>[2x]MGSQSTSNHLWLLSDILGQGATANVFRGRHKKTGDLFAIKVFNNISFLRPVDVQMREFEVLKKLNHKNIVKLFAIEEETTTRHKVLIMEFCPCGSLYTVLEEPSNAYGLPESEFLIVLRDVVGGM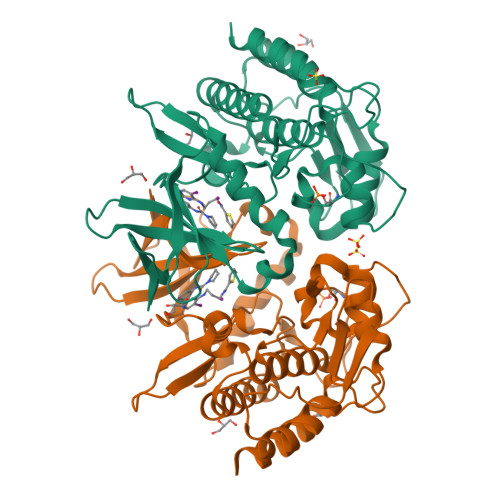NHLRENGIVHRNIKPGNIMRVIGEDGQSVYKLTDFGAARELEDDEQFVSLYGTEEYLHPDMYERAVLRKDHQKKYGATVDLWSIGVTFYHAATGSLPFRPFEGPRRNKEVMYKIITGKPSGAISGVQKAENGPIDWSGDMPVSCSLSRGLQVLLTPVLANILEADQEKCWGFDQFFAETSDILHRGNSHHHHHH> MSMLAKIAKNVVKTQALKNTTAAQTPSFQAPGNQDKILKWISTLSNKATTGESRSYCTQLSSLVSFYNKQHVEQIPTIDFNEWKSVISTQGLVDKVKENYESLIKEQYNTDAISKQISSASSKALDDIEN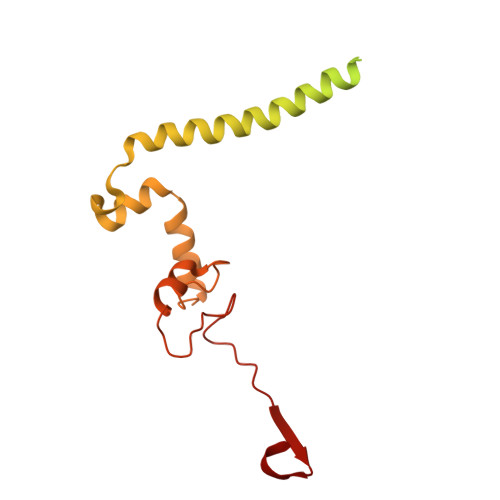ELSFHAAIWLNAYADYTMFLFELEEYNDPNDYLMHENFDFFRGLETELEELTETHNYIPGAKDDVNLRGYLATQFAWGKKVISFYRHPADDFKCAKATKNMLGR> MKRLGKVLHYAKQGFLIVRTNWVPSLNDRVVDKRLQFVGIVKDVFGPVKMPYVAIKPKVSNPEIYVGEVLY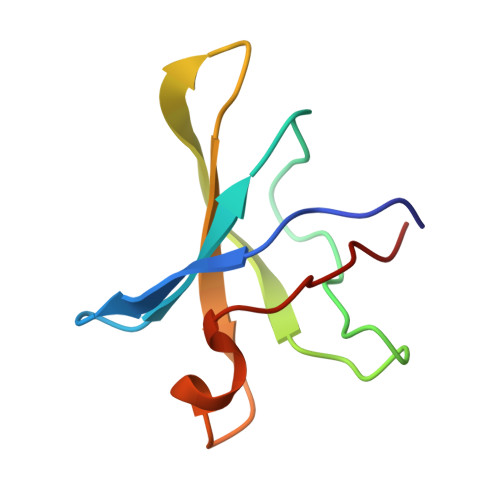VDE> MGSDKIHHHHHHMRILSGMRPTGKLHIGHLVGALENWVKLQEEGNECFYFVADWHALTTHYDDVSKLKEYTRDLVRGFLACGIDPEKSVIFVQSGVKEHAELALLFSMIVSVSRLERVPTYKEIKSELNYKDLSTAGFLIYPVLQAADILIYKAEGVPVGEDQVYHIELTREIARRFNYLYDEVFPEPEAILSRVPKLPGTDGRKMSKSYGNIINLEISEKELEQTILRMMTDPARVRRSDPGNPENCPVWKYHQAFDISEEESKWVWEGCTTASIGCVDCKKLLLKNMKRKLAPIWENFRKIDEDPHYVDDVIMEGTKKAREVAAKTMEEVRRAMNLMF

Tryptophanyl-tRNA synthetase (TrpRS; EC 6.1.1.2) belongs to the class I AARSs and, as its name implies, catalyzes the activation of tryptophan by ATP and the subsequent transfer of the tryptophanyl moiety onto the cognate tRNA. Class I AARSs are mostly monomeric and contain a classic Rossmann nucleotide-fold catalytic domain and two highly conserved sequence motifs ‘HIGH’ and ‘KMSKS’ that are critical for their function. Typically, this enzyme, which is an obligate dimer, binds ATP and l-tryptophan in one subunit, while the tRNA anticodon region is recognized by the TAB domain from the other subunit. Here, we report a novel TrpRS from Thermotoga maritima that contains a [4Fe–4S] cluster bound to the tRNA anticodon-binding domain and an l-tryptophan located in the active site.

The final model contains one TmTrpRS molecule (residues 0–328), one iron–sulfur cluster [4Fe–4S], one tryptophan and 56 water molecules in the asymmetric unit. The N-terminal catalytic domain adopts a canonical Rossmann nucleotide-binding fold (residues 1–181 and 296–328) with a central, five-stranded, parallel β-sheet (β1–β5; the strand order is 32145) and a tRNA anticodon-binding domain that adopts an all-helical fold (residues 187–294). The TAB domain is composed of four α-helices (α11–α14) and two 310 helices (η3 and η4) that are packed as a bundle. Remarkably, the structure of TmTrpRS differs from other TrpRS by the presence of an iron–sulfur cluster [4Fe–4S] in the C-terminal TAB domain. In addition, an l-tryptophan molecule is bound in the active site, which was not expected since tryptophan was not added to any of the reagents used in crystallization or purification. In the TmTrpRS structure, which is similar to the ‘open’ conformation of BsTrpRS, the KMSKS motif is further from the ATP site and is not poised to bind ATP. Accordingly, no ATP molecule was observed in the crystal. Although a single molecule is present in the asymmetric unit, crystal-packing analysis identified a crystallographic dimer that is likely to represent the biologically relevant dimer. In the case of the [4Fe–4S] cluster in TmTrpRS, we believe that it plays a role in the recognition of specifically modified tRNA; however, the biological implications of this are unknown at present.> SNAEQYHSQVVGKIGYIARCMQTIDPENNLKKIREDYQDVLIWAEKNYRFEEILEASKSGKCPNDLDALSRRSLILQELLRLVSSISPFKMKLDLIESQYEKMKQHVNLWKSDYHVKLNQLNQLTDYLKNAAPTPKNNFLRAMTSVLQMQIAQYGITEDNEGINQLFKLGLH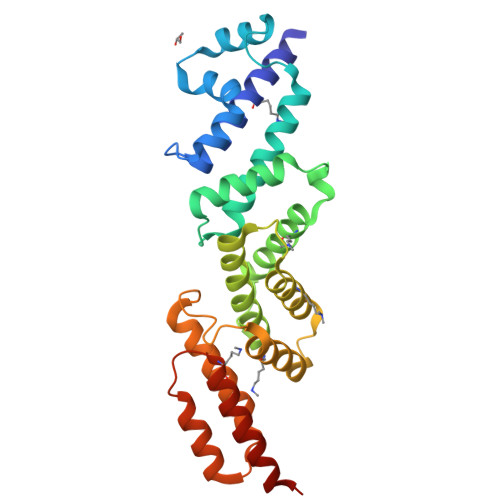LLAMANEKIDEQYHLFKGYVKDQPEESPFEGILPAEDQKILVKTMIDYAMPKLSSKVLQDKLSALSSSDVLTKTLLDSIDRIVKENEKLNALSK>MSGGKYVDSEGHLYTVPIREQGNIYKPNNKAMADELSEKQVYDAHTKEIDLVNRDPKHLNDDVVKIDFEDVIAEPEGTHSFDGIWKASFTTFTVTKYWFYRLLSALFGIPMALIWGIYFAILSFLHIWAVVPCIKSFLIEIQCISRVYSIYVHTVCDPLFEAVGKIFSNVRINLQKEI[11x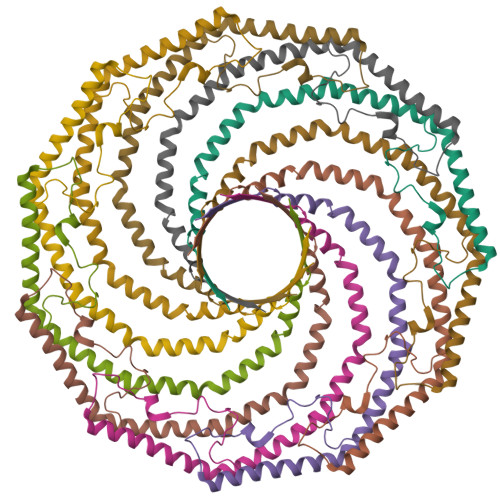]> MATEGMILTNHDHQIRVGVLTVSDSCFRNLAEDRSGINLKDLVQDPSLLGGTISAYKIVPDEIEEIKETLIDWCDEKELNLILTTGGTGFAPRDVTPEATKEVIEREAPGMALAMLMGSLNVTPLGMLSRPVCGIRGKTLIINL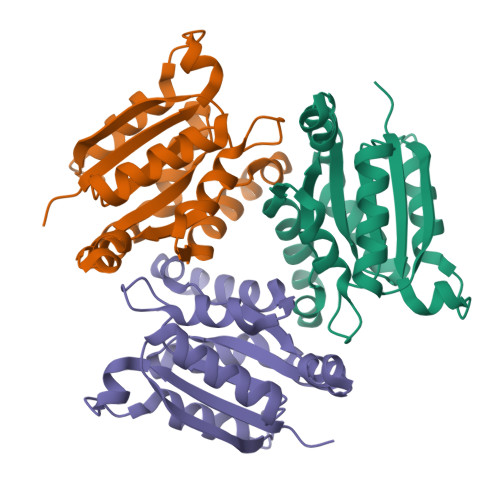PGSKKGSQECFQFILPALPHAIDLLRDAIVKVKEVHDELEDLPS>[4x]GAMVIRDENYFTDKYELTRTHSEVLEAVKVVKPGKT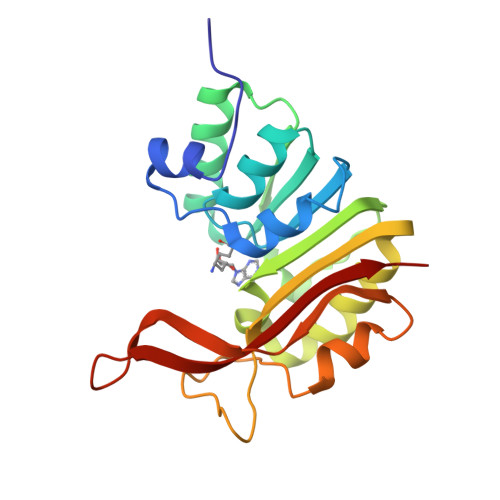LDLGCGNGRNSLYLAANGYDVDAWDKNAMSIANVERIKSIENLDNLHTRVVDLNNLTFDRQYDFILSTVVLMFLEAKTIPGLIANMQRCTKPGGYNLIVAAMDTADYPCTVGFPFAFKEGELRRYYEGWERVKYNEDVGELHRTDANGNRIKLRFATMLARKK> SKLSLSSDQLNHCHQALGVFRGKIQNPDSIAHEFTGLQANRMWPSELLLNSTVAMNSVNVEKNRYSDVVPFDKNRIVLNPCKDSSAKGYVNASLIKTSESESISQFIATQGPLPHTMEDFWEMVIQQHCPIIVMLTRLVDNNRTVKCGDYFQDEDGPREFGNISLTTKWIKTTDTSLMLRNLEVNYKETEDQPMSVLHIQYPEWPDHGVPKDTVAVREILKRLYQVPPSLGPIIVHCSAGIGRTGTYC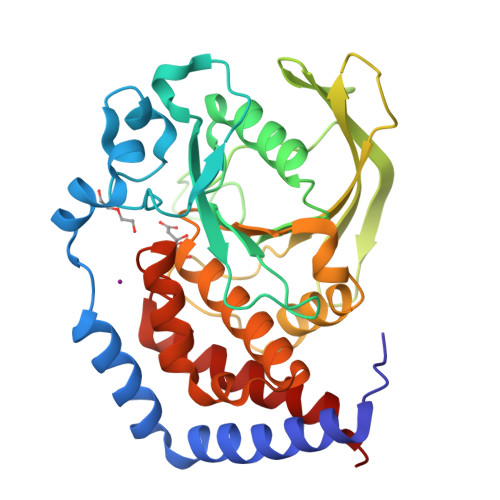AIHNTIQRILAGDMSALDLAKTVALFRKQRIGMVQTMDQYFFCYNAIVDELEDLTAGT>[4x]GMTDIPDRKEAVISLWPEFAKAIVSGKKTVEFRRRIPLPALSARIWIYATRPVKSVIGFAYLEAIVQGDVNTLWSRYGREAFLSEQQYRDYFEGTEKATAFLLRDHQPIRPINLDQLKEIRANFQPPQSLTWLRKEETQKLVSLTSQVE

In the ethanologenic bacterium Zymomonas mobilis ZM4, the gene ZMO0922 encodes a 148 amino acid polypeptide, which has been annotated as a putative ASCH domain-containing protein (ZmASCH) that belongs to family 23. Here, we report the three-dimensional crystal structure of ZmASCH which confirms the fold of a central β-barrel core and reveals a positively-charged cleft with a pocket on the surface. In vitro assays showed that ZmASCH bound nucleic acids and possessed cleavage activity specifically towards single-stranded RNAs. The weak nuclease activity of ZmASCH depended on magnesium ions and the protein appeared to prefer the consecutive pyrimidine-adenine dinucleotides for its cleavage activity.

The structure of ZmASCH protein comprises five α-helices and a six-stranded β-sheet, the latter forming the central β-barrel. This β-barrel is flanked by two pairs of antiparallel α-helices (α2/α3 and α4/α5) as well as the single helix α1. There are two and four protein molecules in the asymmetric unit of the trigonal and monoclinic crystal forms, respectively. The conformations of individual monomers are in excellent agreement, and all monomers superimpose with RMSD values of less than 0.3 Å, with the largest deviations in the loops between strands β2 and β3 and helices α4 and α5. As the ssRNA-cleavage activity of ZmASCH was dependent on magnesium ions, but inhibited by other transition metal ions, such as zinc or cobalt, co-crystallization of the wild-type protein with either ZnCl2 or CoCl2 was attempted. However, we could not locate any bound transition metal ions in either crystal form, suggesting that high affinity binding of the metal ion to the protein molecule is probably accomplished in the presence of a nucleic acid.>SGVGHSTGNYNNRTIFHYHGDEVTIICHATRHIHLNMSPTEEYKIYDTNHGPEFPNTGDQTQQGRNTVNDSYHAKVETPWYLINPNSWGIWFNPADFQQLITTCTHVTIETLTQEIDNIVIKTVSKQGSGAEETTQYNNDLTALLEVALDKSNMLPWVADNMYLNSLGYIPWRPCKLTQFCYHTNFYNTINLLEGTQQNQWSQIKEGIQYDNLQFTPIET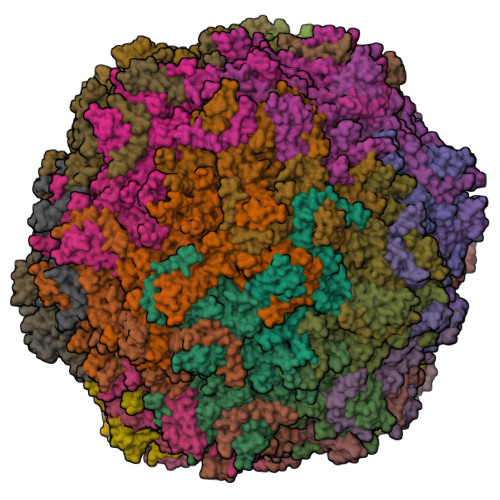SAEIDLLRTGDSWTSGTYHFKCKPTQLFYHWQSTRHIGAPHPTTSPEQEGQKGQIIQDTNGWQWGDRDNPISASTTVKDFHIGYSWPEWRWHYSTGGPSINPGSAFSQTPWGSEVGGTRLTQGASEKAIFDYNHGEAEPGHRDQWWQNNAQQTGQTNWAIKNAHQSELRNATASRETFWTQDYHNTFGPYTAVDDVGIQYPWGAMWGKQPDTTHKPMMSAHAPFTCQNGPPGQLLVKLAPNYTDSLNNEGLQTNRIVTFATFWWTGRCTFKAKLRTPRQFNAYQLPGIPSGTNPKKFVPDAIGRFELPFMPGRAMPNYTY[60x]> XDPATIMCRAAADTCTFF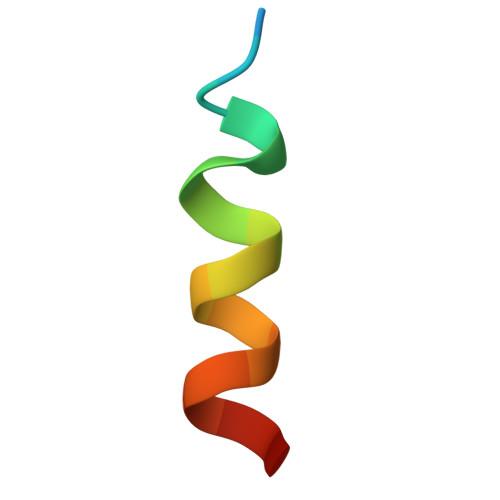X> XSGRGKGG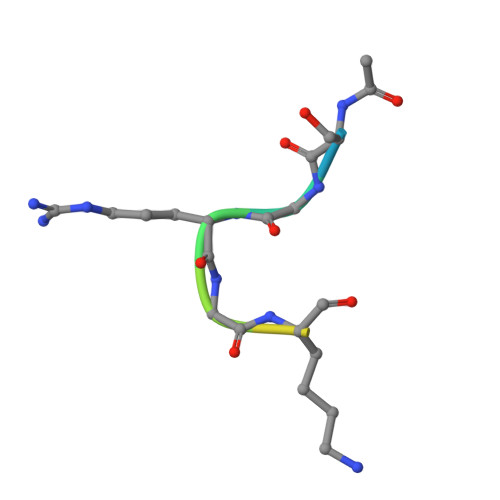KGL>ETGPHMFWTGWGPWERCTAQCGGGIQARRRICENGPDCAGCNVEYQSCNTNPCPELKKTTPWTPWTPVNISDNGGHYEQRFRYTCKARLADPNLLEVGRQRIEMRYCSSDGTSGCSTGTLEVL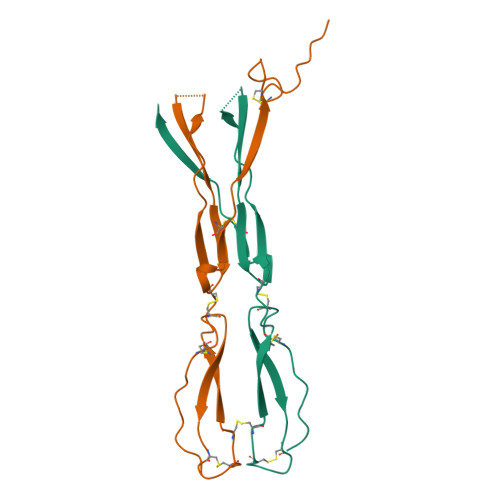FQ[2x]> GPHMAQGTLIRVTPEQPTHAVCVLGTLTQLDICSSAPEDCTSFSINASPGVVVDIAHGPPAKKKSTGSSTWPLDPGVEVTLTMKVASGSTGDQKVQISYYGPKTPPVKALLYLTGVEISLCADITRTGKVKPTRAVKDQRTWTWGPCGQGAILLVNCDRDNLESSAMDCEDDEVLDSEDLQDMSLMTLSTKTPKDFFTNHTLVLHVARSEMDKVRVFQATRGKLSSKCSVVLGPKWPSHYLMVPGGKHNMDFYVEALAFPDTDFPGLITLTISLLDTSNLELPEAVVFQDSVVFRVAPWIMTPNT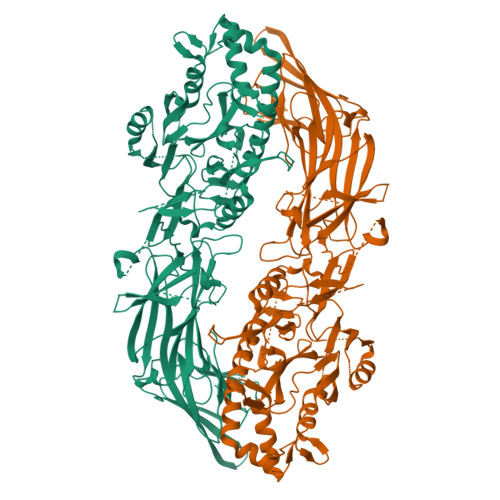QPPQEVYACSIFENEDFLKSVTTLAMKAKCKLTICPEEENMDDQWMQDEMEIGYIQAPHKTLPVVFDSPRNRGLKEFPIKRVMGPDFGYVTRGPQTGGISGLDSFGNLEVSPPVTVRGKEYPLGRILFGDSCYPSNDSRQMHQALQDFLSAQQVQAPVKLYSDWLSVGHVDEFLSFVPAPDRKGFRLLLASPRSCYKLFQEQQNEGHGEALLFEGIKKKKQQKIKNILSNKTLREHNSFVERCIDWNRELLKRELGLAESDIIDIPQLFKLKEFSKAEAFFPNMVNMLVLGKHLGIPKPFGPVINGRCCLEEKVCSLLEPLGLQCTFINDFFTYHIRHGEVHCGTNVRRKPFSFKWWNMVP> MNNDNPLFKSAMVA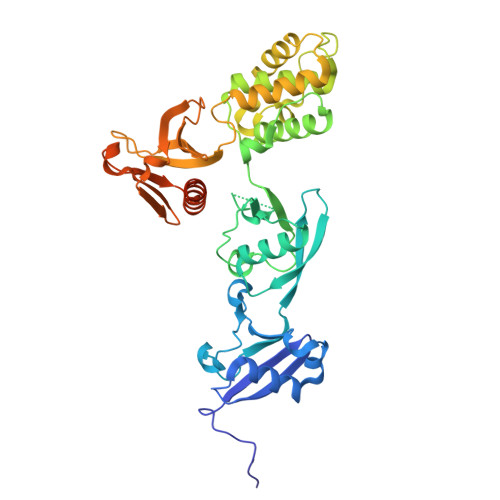LSLKISIGNVVKTMQFEPSTMVYDACRMIRERIPEALAGPPNDFGLFLSDDDPKKGIWLEAGKALDYYMLRNGDTMEYRKKQRPLKIRMLDGTVKTIMVDDSKTVTDMLMTICARIGITNHDEYSLVRELMEEKKDELNWLDHGRTLREQGVEEHETLLLRRKFFYSDQNVDSRDPVQLNLLYVQARDDILNGSHPVSFDKACEFAGFQCQIQFGPHNEQKHKAGFLDLKDFLPKEEVKQKGERKIFQAHKNCGQMSEIEAKVRYVKLARSLKTYGVSFFLVKEKMKGKNKLVPRLLGITKECVMRVDEKTKEVIQEWSLTNIKRWAASPKSFTLDFGDYQDGYYSVQTTEGEQIAQLIAGYIDIILKKKKSKDHFGLEGDEESTMLEDSVSPKKST>APGLRPQSYTLQVHEEDQDVERSQVRSAAQQSTWRDFGRKLRLLSGYLWPRGSPALQLVVLICLGLMGLERALNVLVPIFYRNIVNLLTEKAPWNSLAWTVTSYVFLKFLQGGGTGSTGFVSNLRTFLWIRVQQFTSRRVELLIFSHLHELSLRWHLGRRTGEVLRIADRGTSSVTGLLSYLVFNVIPTLADIIIGIIYFSMFFNAWFGLIVFLCMSLYLTLTIVVTEWRTKFRRAMNTQENATRARAVDSLLNFETVKYYNAESYEVERYREAIIKYQGLEWKSSASLVLLNQTQNLVIGLGLLAGSLLCAYFVTEQKLQVGDYVLFGTYIIQLYMPLNWFGTYYRMIQTNFIDMENMFDLLKEETEVKDLPGAGPLRFQKGRIEFENVHFSYADGRETLQDVSFTVMPGQTLALVGPSGAGKSTILRLLFRFYDISSGCIRIDGQDISQVTQASLRSHIGVVPQDTVLFNDTIADNIRYGRVTAGNDEVEAAAQAAGIHDAIMAFPEGYRTQVGERGLKLSGGEKQRVAIARTILKAPGIILLDEATSALDTSNERAIQASLAKVCANRTTIVVAHRLSTVVNADQILVIKDGCIVERGRHEALLSRGGVYADMWQLQQGQEETSEDTKPQTMER[2x];>ECECG[2x]

ATP-binding cassette transporter B6 (ABCB6), a protein essential for heme biosynthesis in mitochondria, also functions as a heavy metal efflux pump. ATP-binding cassette transporter B6 (ABCB6) is a homodimeric Type IV half-transporter comprising a single transmembrane domain (TMD) and a nucleotide-binding domain (NBD) with an N-terminal extension (TMD0). The TMD is responsible for substrate recognition and translocation, while the NBD is involved in ATP binding and hydrolysis, providing the energy required for substrate transport. In the present study, we determined cryo-electron microscopy (cryo-EM) structures of human ABCB6 in complex with a Cd(II) ion, which is coordinated by two molecules of either GSH or PC2, at resolutions of 3.2 and 3.1 Å, respectively.

Interestingly, the stimulatory effect of Cd(II) on hABCB6core activity was also observed when PC2 was present, resembling the response seen with GSH. The structures of hABCB6core in complex with Cd(II) and GSH (or PC2) are shaped like a lassical inward-facing transporter in which the substrate-binding cavity within the TMD region is open towards the cytoplasm. Superimposition indicates that the two structures are nearly identical, with a Cα root-mean-square deviation (r.m.s.d.) of 0.6 Å. The overall binding mode of Cd(II) with PC2 in hABCB6core is very similar to that of Cd(II) with GSH, although the molecular basis of complex formation differs. Specifically, the two cysteine residues of each PC2 molecule participate in Cd(II) coordination to form a tetrathiolate. The glycyl unit at the C-terminus does not participate in interactions with nearby residues and remains freely exposed within the binding cavity. Although human ABCB6 in vivo would not encounter PC2, which is primarily found in plant and certain fungal cells, the high conservation of the mode of complex formation and the residues involved in binding GSH and PC2 suggests that ABCB6/HMT-1/Atm1-like transporters share a common evolutionary origin and mechanism for heavy metal binding and export across diverse organisms. The CASTp program calculated that the cavity volumes of the Cd(II)-bound structures in complex with GSH and PC2 to be approximately 2312 Å3 and 2573 Å3, respectively. The smallest tilt difference of 3.9° is observed between the apo and Cd(II):GSH (or PC2)-bound states, with a clockwise rotation of one NBD with respect to the other NBD.>AVGPVADLTVTNANIVPDGFERAAIVVNNVFPAPLITGNMGDNFQLNLVNQMTNHTMLKTTSIHWHGFFQKGTNWADGPAFINQCPIASGNSFLYDFQVPGQAGTFWYHSHLSTQYCDGLRGPFVVYDPNDPHANLYDVDDESTVITLADWYHVAAKLGPRFPKGADSTLINGLGRSTSTPTADLAVISVTKGKRYRFRLVSLSCDPNYTFSIDSHQLTVIEADGVSTQPVTVDSIQIFAAQRYSFVLNANQDVDNYWIRANPNFGTTGFADGVNSAILRYDDADPVEPVTNQTGTTLLLETDLHPLTSMPVPGNPTQGGADLNLNMAFNFDGTNFFINGESFTPPTVPVLLQIISGANTAQDLLPSGSVYSLPSNSSIEITFPATTAAPGAPHPFHLHGHVFAVVRSA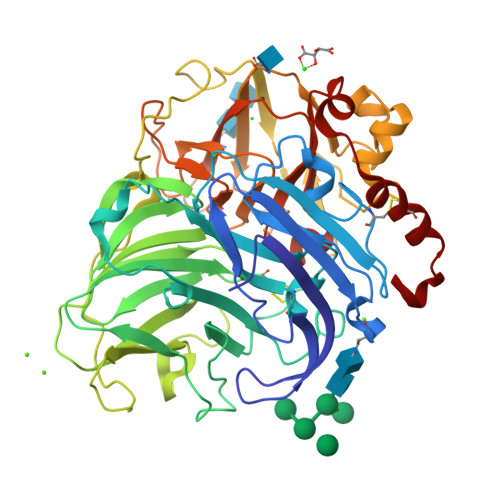GSTSYNYDDPVWRDVVSTGTPQAGDNVTIRFQTDNPGPWFLHCHIDFHLDAGFAVVMAEDIPNTVNANPVPQAWSNLCPTYDALEPSNE[2x]Bacteriophage T5, a representative member of the T5-like family of siphophages, serves as an excellent model for studying the assembly, infection, cell wall perforation, and DNA ejection mechanisms of this phage family. In this study, we used cryo-electron microscopy (cryo-EM) to determine the structures of mature T5 (a laboratory-adapted, fiberless T5 mutant) and urea-treated empty T5 (lacking the tip complex) at near-atomic resolutions. The T5 head comprises 775 copies of MCP gp8, arranged into 11 pentons and 120 hexons, forming an icosahedral shell with a triangle number (T) of 13. The T5 tail, which comprises 40 trimeric rings of the TTP and a distal tip complex, is connected to a unique five-fold vertex of the head by the connector complex.

Using the local reconstruction method, we then obtained the structures of the connector complex and the portal of mature T5 at resolutions of 4.8 and 3.2 Å, respectively. The connector complex comprises two dodecameric portal protein pb7 and adaptor protein p144, and a hexameric tail terminator protein p142. We also built an atomic model of T5 terminator protein p142, including all 161 amino acid residues. The tail terminator comprises six copies of protein p142. Each p142 contains two α-helices and a β-barrel structure facing the lumen of the tube, which are homologous to the terminator proteins of other phages, such as Lambda (gpU) and SPP1 (gp17). As observed for the T5 adaptor, substantial conformational changes occur in the C-terminus between two adjacent p142 monomers, which primarily mediate the structural symmetry mismatch between the six-fold symmetric tail terminator and the three-fold symmetric TTP. Furthermore, the contact interface between the DNA and TMP was observed within the lumen of the adaptor-terminator channel. In contrast, in the T5 connector, DNA may interact with multiple regions to prevent its release, including the negative electrostatic potential inside the connector channel and the presence of TMP in the tail tube, as previously proposed for phage DT57C. The pairwise interfaces between the protein components of the T5 connector complex and the TTP are complementary in terms of electrostatic potential energy. In the mature state, the negative electrostatic potential inside the connector channel and TMP collectively prevent the release of DNA.

>MDHRTSIAQAMVDRISKQMDGSQPDEYFNNLYGNVSRQTYKFEEIREFPYVAVHIGTETGQYLPSGQQWMFLELPILVYDKEKTDIQEQLEKLVADIKTVIDTGGNLEYTVSKPNGSTFPCEATDMIITSVSTDEGLLAPYGLAEINVTVRYQPPRRSLRR[6x]>MGRAHKETLDKLTNAAINKINLLNTSKVKYLVSSAFAGLYVGIGILLIFTIGGLLTDAGSPMTKIVMGLSFAIALSLVIMTGTEVFTGNNMVMSAGMLNKGVSIKDTSKIWAYSWVGNLIGALVLGIIFVGTGLVDKGPVAEFFANTAASKASMPFTALFFRGILCNILVCVSVLCSFRTNSDTAKIIMIFLCLFAFITSGFEHSVANMTIYSVSLFSPTISTVTIGGAIYNLVAVTLGNIVGGALFMGLGTYILGKEKLNAAAE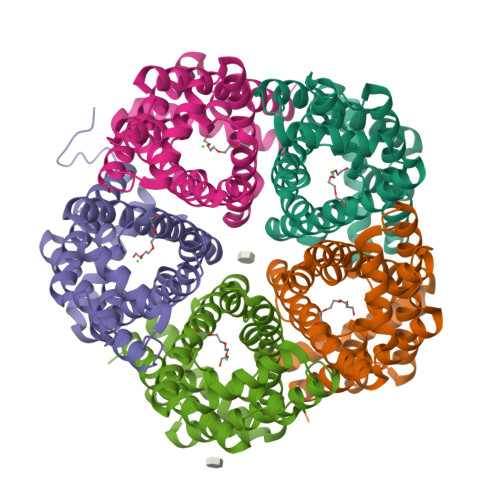NLY[5x]> DEFQWKGLPVVKSGLDVGGMPTGTRYH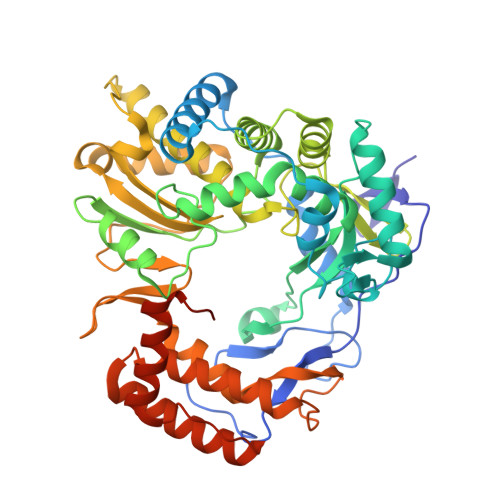RSPAWPEEQPGETHAPAPFGSGDKRYTFSQTEMLVNGLKPYTEPTAGVPPQLLSRAVTHVRSYIETIIGTHRSPVLTYHQACELLERTTSCGPFVQGLKGDYWDEEQQQYTGVLANHLEQAWDKANKGIAPRNAYKLALKDELRPIEKNKAGKRRLLWGCDAATTLIATAAFKAVATRLQVVTPMTPVAVGINMDSVQMQVMNDSLKGGVLYCLDYSKWDSTQNPAVTAASLAILERFAEPHPIVSCAIEALSSPAEGYVNDIKFVTRGGLPSGMPFTSVVNSINHMIYVAAAILQAYESHNVPYTGNVFQVETIHTYGGDCMYSVCPATASIFHTVLANLTSYGLKPTAIKPTNTPVFLKRTFTQTPHGIRALLDITSITRQFYWLKANRTSDPSSPPAFDRQARSAQLENALAYASQHGPVMFDTVRQIAIKTAQGEGLVLVNTNYDQALATYNAWFIGGTPDPVGHTEGTHKIVFEME>[24x]MIPQTLTNTNLFIDGVSFAGDVPSLTLPKLAVKTEQYRAGGMDAPVSIDMGLEAMEAKFSTNGARREALNFFGLADQSAFNGVFRGSFKGQKGASVPVVATLRGLLKEVDPGDWKAGEKAEFKYAVAVSYYKLEVDGREVYEIDPVNGVRAINGVDQLAGMRNDLGL;>[6x]MPEQAVTLEALYAAIEQVLRERLPEAQLIGFWPGVPENTPAVSLEIAELLPERDPGTGESALLCRLQARIMVPPGADRQAVSIACGIVRTLREQTWNLSLQPARFVRSAVDGSREELKSLRVWLVEWTQSLRLGDPEWAWEDQPPGSLMLGFDPQTGPGHEPDYFAPEALA;>MSFF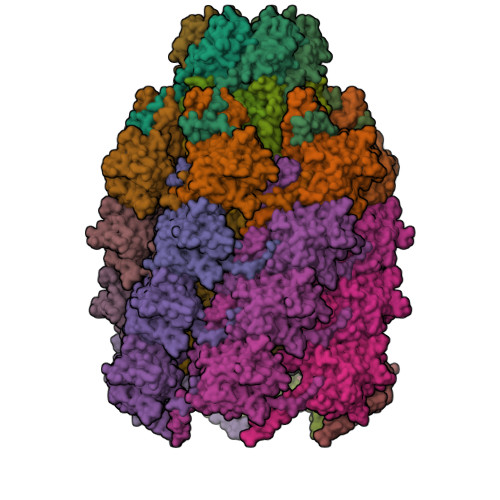HGVTVTNVDIGARTIALPASSVIGLCDVFTPGAQASAKPNVPVLLTSKKDAAAAFGIGSSIYLACEAIYNRAQAVIVAVGVETAETPEAQASAVIGGISAAGERTGLQALLDGKSRFNAQPRLLVAPGHSAQQAVATAMDGLAEKLRAIAILDGPNSTDEAAVAYAKNFGSKRLFMVDPGVQVWDSATNAARNAPASAYAAGLFAWTDAEYGFWSSPSNKEIKGVTGTSRPVEFLDGDETCRANLLNNANIATIIRDDGYRLWGNRTLSSDSKWAFVTRVRTMDLVMDAILAGHKWAVDRGITKTYVKDVTEGLRAFMRDLKNQGAVINFEVYADPDLNSASQLAQGKVYWNIRFTDVPPAENPNFRVEVTDQWLTEVLDVA[24x]> CUGCUGGCUAAGGCAUGAAAGUGCUAU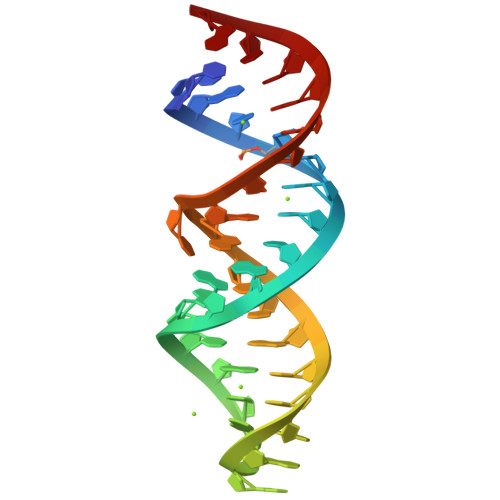GCCUGCUG>[3x]MTTPPLLQLPVEVKKTELNGFWDTGAQITCIPEAFLKEEIPIGEAQIKTLHGTKLQSVYYLKFKVLGRKVEAEVTTSPFDYVIISPSDIPWYKPQPLELTVKLPVQDFKKELINKANINNEEKKQLAKLLDKYDVLWQQWENQVGHRKIP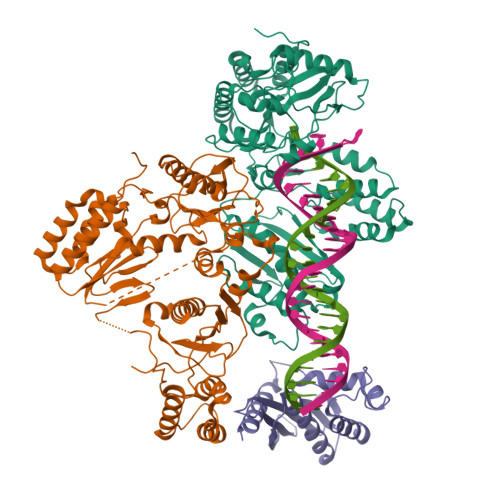PHNIATGTVAPRPQRQYHINTKAKPSIQQVIDDLLKQGVLIKQTSVMNTPIYPVPKPDGKWRMVLDYRAVNKTVPLIGAQNQHSLGILTNLVRQKYKSTIDLSNGFWAHPITKDSQWITAFTWEGKQHVWTRLPQGFLNSPALFTADVVDLLKNIPGISVYVDDIYFSTETVSEHLKILEKVFKILLEAGYIVSLKKSALLRYEVTFLGFSITQTGRGLTSEFKDKIQNITSPRTLKELQSILGLFNFARNFVPNFSEIIKPLYSLISTAEGNNIKWTSEHTRYLEEIVSALNHAGNLEQRDNESPLVVKLNASPKTGYIRYYNKGGQKPIAYASHVFTNTELKFTPLEKLLVTMHKALIKAIDLALGQPIEVYSPIISMQKLQKTPLPERKALSTRWITWLSYLEDPRITFYYDKTLPDLKNVPETVTDKKPKMLPIIEYAAVFYTDGSAIRSPDKNKSHSSGMGIVHAVFKPELTIEHQWSIPLGDHTAQYAEISAVEFACKKANNISGPVLIVTDSDYVARSVNEELPFWRSNGFVNNKKKPLKHISKWKNISDSLLLKRDIIIVHEPGHKPSYTSIHTQGNNLADKLATQGSYTVNNI>[2x]VTAYEEIVCQVFAAVLDRSDVTADADFFALGGHSLLSLRVVARLRALLGVDVGVRDLFEAPTPAALAARLTTQTGRRPAVTRRGPDAPPVLSHFQR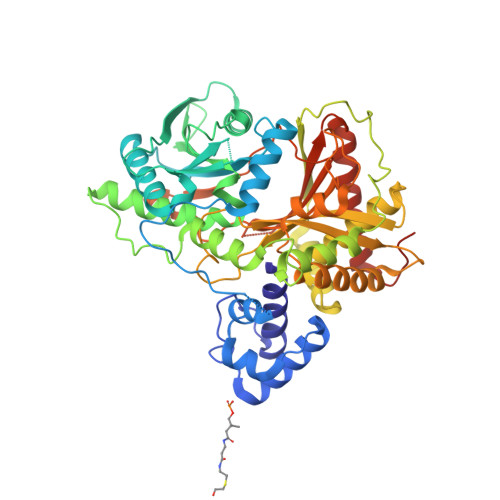GLWLIEQVYQTRGAYNVPLAVHVSDRLDLDVLRAAVRDLVARHEVLRTLVRSSDDGPDPVLLAPEDAAVDVAEVQAAGPVADLLAELTAQPFDLATQIPLRVRMITGEQVDGCVLLLVCHHIAADEWSFAPLLRDLDTAYRARAAGRAPDWEPLPAQYSDYAATLHDWLGEATDPASPLRRQLDYWQHALQDLPDELDLPTDRPRPATASHRGGLARAELPPELVEAVRRLAAQHGVTVFMVVQAAVAVLLHRLGAGDDIPLGSPVADRADEAVHDTVGFFLNTLVLRVNLSGNPTFADLLDRVRAVDLEAFARADAPFDAVVDTVKPPRAVSRHPLFQTMVSYQRRPSDVDRLFGAATRLVEVPLDTAKFDLEFAFIEDGHGGAHIALNYAADLFDHDSAEQLVARLRTVLEHACADPCRPVAGVEVVSGA> 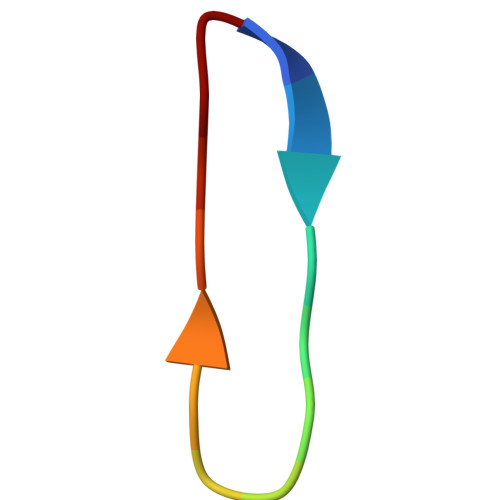VLQLTLGNSTITTQ> MDFLSNFLTDFVGQLQSPTLAFLIGGMVIAALGTQLVIPEAISTIIVFMLLTKIGLTGGMAIRNSNLTEMLLPVAFSVILGILIVFIARFTLAKLPNVRTVDALATGGLFGAVSGSTMAAALTTLEESKISYEAWAGALYPFMDIPALVTAIVVANIYLNKRKRKSAAASIEESFSKQPVAAGDYGDQTDYPRTRQEYLSQQE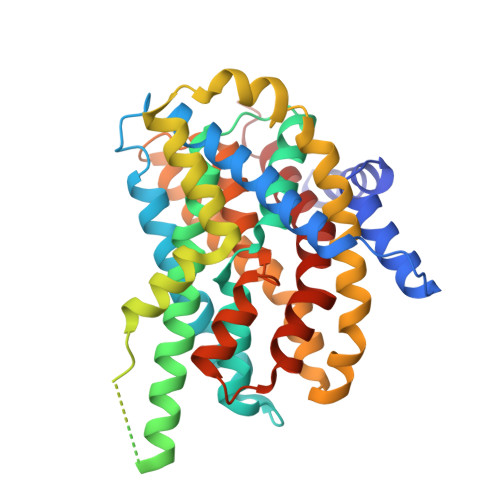PEDNRVKIWPIIEESLQGPALSAMLLGLALGIFTKPESVYEGFYDPLFRGLLSILMLIMGMEAWSRIGELRKVAQWYVVYSLIAPIVHGFIAFGLGMIAHYATGFSLGGVVVLAVIAASSSDISGPPTLRAGIPSANPSAYIGSSTAIGTPIAIGVCIPLFIGLAQTLGAG> MAHHHHHHVDDDDKMVTDQRWLIDKSALVRLTDSPDMEIWSNRIERGLVHITGVTRLEVGFSAECGEIARREFREPPLSAMPVEYLTPRIEDRALEVQTLLADRGHHRGPSIPDLLIAATAELSGLTV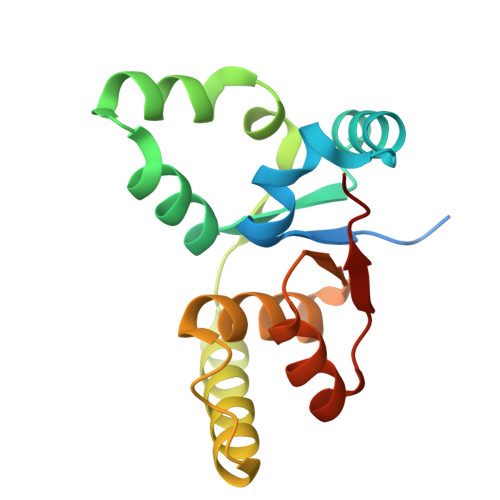LHVDKDFDAIAALTGQKTERLTHRPPSA> QKPGETKEVHPQLTTFRCTKRGGCKPATNFIVLDSLSHPIHRAEGLGPGGCGDWGNPPPKDVCPDVESCAKNCIMEGIPDYSQYGVTTNGTSLRLQHILPDGRVPSPRVYLLDKTKRRYEMLHLTGFEFTFDVDATKLPCGMNSALYLSEMHPTGAKSKYNPGGAYYGTGYCDAQCFVTPFINGLGNIEGKGSCCNSMDIWEANSRASHVAPHTCNKKGLYLCEGEECAFEGVCDKNGCGWNNYRVNVTDYYGRGEEFKVNTLKPFTVVTQFLANRRGKLEKIHRFYVQDGKVIESFYTNKEGVPYTNMIDDEFCEATGSRKYMELGATQGMGE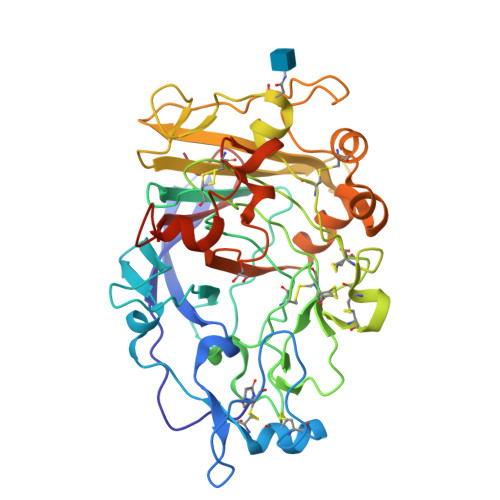ALTRGMVLAMSIWWDQGGNMEWLDHGEAGPCAKGEGAPSNIVQVEPFPEVTYTNLRWGEIGSTYQELQ>MADNLPSDFDVIVIGTGLPESIIAAACSRSGQRVLHVDSRSYYGGNWASFSFSGLLSWLKEYQENNDVVTENSMWQEQILENEEAIPLSSKDKTIQHVEVFCYASQDLHKDVEEAGALQKNHASVTSAQSAEAAEAAETSCLPTAVEPLSMGSCEIPAEQSQCPGPESSPEVNDAEATGKKENSDAKSSTEEPSENVPKVQDNTETPKKNRITYSQIIKEGRRFNIDLVSKLLYSRGLLIDLLIKSNVSRYAEFKNITRILAFREGTVEQVPCSRADVFNSKQLTMVEKRMLMKFLTFCVEYEEHPDEYRAYEGTTFSEYLKTQKLTPNLQYFVLHSIAMTSETTSCTVDGLKATKKFLQCLGRYGNTPFLFPLYGQGELPQCFCRMCAVFGGIYCLRHSVQCLVVDKESRKCKAVIDQFGQRIISKHFIIEDSYLSENTCSRVQYRQISRAVLITDGSVLRTDADQQVSILTVPAEEPGSFAVRVIELCSSTMTCMKGTYLVHLTCMSSKTAREDLERVVQKLFTPYTEIEAENEQVEKPRLLWALYFNMRDSSDISRDCYNDLPSNVYVCSGPDSGLGNDNAVKQAETLFQQICPNEDFCPAPPNPEDIVLDGDSSQQEVPESSVTPETNSETPKESTVLGNPEEP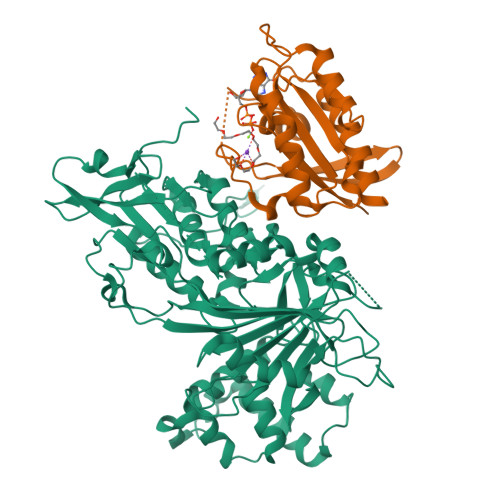SE[4x];>MTSRKKVLLKVIILGDSGVGKTSLMNQYVNKKFSNQYKATIGADFLTKEVMVDDRLVTMQIWDTAGQERFQSLGVAFYRGADCCVLVFDVTAPNTFKTLDSWRDEFLIQASPRDPENFPFVVLGNKIDLENRQVATKRAQAWCYSKNNIPYFETSAKEAINVEQAFQTIARNALKQETEVELYNE[4x]PRDM (PRDI-BF1 and RIZ homology domain containing) proteins comprise a distinct branch of known and putative protein lysine methyltransferases (PKMTs). All PRDMs contain an N-terminal PR domain that shares the canonical SET domain methyltransferase fold, but with only 20–30% amino acid sequence identity. The human PRDM9 protein consists of an N-terminal Krüppel associated box (KRAB) domain, a nuclear localization signal, an SSXRD motif, a pre-SET zinc-knuckle motif preceding the PR domain, followed by one post-SET and a distal array of 13 zinc-finger motifs at the C-terminus. Biochemical characterization of PRDM9 catalytic activity with a histone peptide (residues 1–25 of H3) as an in vitro substrate indicated that PRDM9 is the most active histone methyltransferase characterized in vitro, trimethylating H3K4me2 with a kcat value of 18,000 ± 900 h−14.

To better understand the molecular interaction between PRDM9 and MRK-740 and mechanism of inhibition, we determined the crystal structure of the PRDM9 catalytic domain (residues 195–385) in a ternary complex with SAM and MRK-740 at 2.58 Å resolution. Clear electron density for MRK-740 was located adjacent to the SAM-binding site and allowed unambiguous placement of the inhibitor molecule. An analysis of the intermolecular contacts revealed a network of largely hydrophobic interactions between PRDM9 side chains and MRK-740. Additionally, the pyridine ring of MRK-740 forms a π-stacking interaction with W356. The pyridine nitrogen is presumed to be protonated due to the basicity of the isolated 4-aminopyridine group (pKa = 9.2) and forms a long-range electrostatic interaction with the sidechain of Asp325. Significant additional interactions were observed between the adenosine moiety of SAM and the two central rings of MRK-740. Collectively, the extensive interaction surface between SAM and MRK-740 explains why we observed SAM-dependent inhibition. The binding position of the substrate lysine is sterically occluded by both methoxy groups of the MRK-740 benzene ring. In the MRK-740-bound protein, the substrate recognition helix is flipped in the opposite direction, thereby preventing the enzymatically active conformation seen in the mouse structure. Taken together, the structural data are consistent with our biochemical results indicating a SAM-dependent, peptide-competitive mechanism of action (MOA) for MRK-740.

>[2x]SEPQDDDYLYCEMCQNFFIDSCAAHGPPTFVKDSAVDKGHPNRSALSLPPGLRIGPSGIPQAGLGVWNEASDLPLGLHFGPYEGRITEDEEAANNGYSWLITKGRNCYEYVDGKDKSWANWMRYVNCARDDEEQNLVAFQYHRQIFYRTCRVIRPGCELLVWYGDEYGQELGIKWGSKWKKELMAGREPKP> GRFGKYGGQYVPETLMPALEELEEAYERAKNDPEFQAELEYYLRDYVGRPTPLYFAENLTKD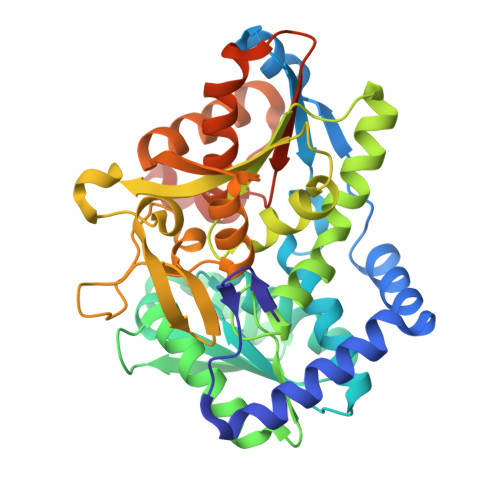LGGAKIYLKREDLNHTGAHKINNALGQALLAKRMGKKRVIAETGAGQHGVATATVAAMFGLECVVYMGAEDIERQALNVFRMKLLGAKVRPVTSGSRTLKDAINEAMRDWVTNVEDTFYIIGSVVGPHPYPMMVRDFQSVIGEEARQQILEKEGRLPDAIVACVGGGSNAMGIFHPFIDDESVRLIGVEAAGKGIETGKHAATLSAGRPGVLHGAMTYLLQDEDGQIIEAHSISAGLDYPGVGPEHAYLKDTGRAEYVSVTDDEALEAFQLLSRTEGIIPALESSHAVAYAMKLAPELSKDQIIVVNLSGRGDKDVNTVARYLLGVELDLEHHHHHH>MSSLSNASHLMEDVQGIRKAQRADGTATVMAIGTAHPPHIFPQDTYADFYFRATNSEHKVELKKKFDRICKKTMIGKRYFNYDEEFLKKYPNITSFDEPSLNDRQDICVPGVPALGAEAAVKAIAEWGRPKSEITHLVFCTSCGVDMPSADFQCAKLLGLRTNVNKYCVYMQGCYAGGTVMRYAKDLAENNRGARVLVVCAELTIIGLRGPNESHLDNAIGNSLFGDGAAALIVGSDPIIGVEKPMFEIVCAKQTVIPNSEDVIHLHMREAGLMFYMSKDSPETISNNVEACLVDVFKSVGMTPPEDWNSLFW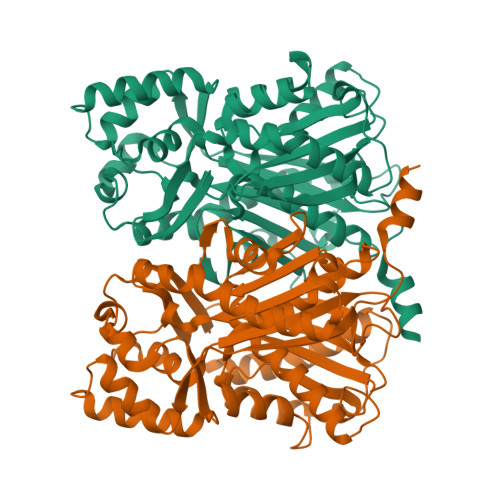IPHPGGRAILDQVEAKLKLRPEKFRATRTVLWDCGNMVSACVLYILDEMRRKSADEGLETYGEGLEWGVLLGFGPGMTVETILLHSLPLM[4x]>LPRPIRNLEVKFTKIFINNEWHESKSGKKFATCNPSTREQICEVEEGDKPDVDKAVEAAQVAFQRGSPWRRLDALSRGRLLHQLADLVERDRATLAALETMDTGKPFLHAFFIDLEGCIRTLRYFAGWADKIQGKTIPTDDNVVCFTRHEPIGVCGAITPWNFPLLMLVWKLAPALCCGNTMVLKPAEQTPLTALYLGSLIKEAGFPPGVVNIVPGFGPTVGAAISSHPQINKIAFTGSTEVGKLVKEAASRSNLKRVTLELGGKN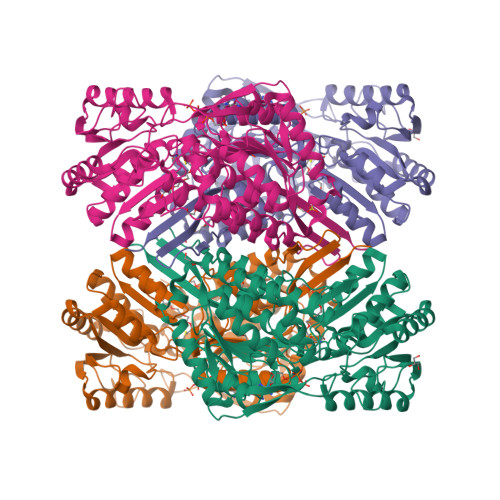PCIVCADADLDLAVECAHQGVFFNQGQCCTAASRVFVEEQVYSEFVRRSVEYAKKRPVGDPFDVKTEQGPQIDQKQFDKILELIESGKKEGAKLECGGSAMEDKGLFIKPTVFSEVTDNMRIAKEEIFGPVQPILKFKSIEEVIKRANSTDYGLTAAVFTKNLDKALKLASALESGTVWINCYNALYAQAPFGGFKMSGNGRELGEYALAEYTEVKTVTIKLG[2x]>AGFSMDKANSEACRDGLRAVMECRNVTHLLQQELTEAQKGFQDVEAQAATCNHTVMALMASLDAEKAQGQKKVEELEGEITTLNHKLQDASAEVERLRR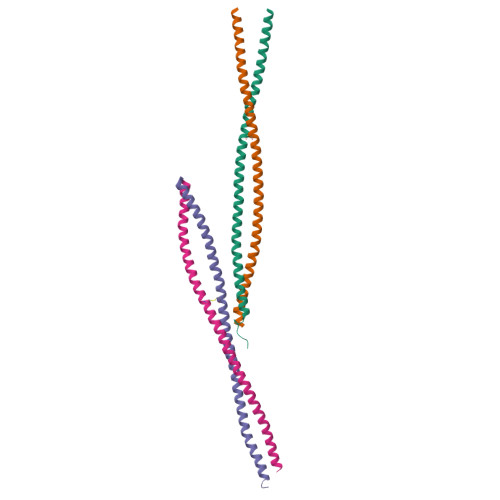ENQVLSVRIADKKYYPSSQDSS[4x]>GPMTDWPVYHRIDGPIVMIGFGSIGRGTLPLIERHFAFDRSKLVVIDPSDEARKLAEARGVRFIQQAVTRDNYRELLVPLLTAGPGQGFCVNLSVDTSSLDIMELARENGALYIDTVVEPWLGFYFDPDLKPEARSNYALRETVLAARRNKPGGTTAVSCCGANPGMVSWFVKQALVNLAADLGVTGEEPTTREEWARLAMDLGVKGIHIAERDTQRASFPKPFDVFVNTWSVEGFVSEGLQPAELGWGTFERWMPDNARGHDSGCGAGIYLLQPGANTRVRSWTPTAMAQYGFLVTHNESISIADFLTVRDAAGQAVYRPTCHYAYHPCNDAVLSLHEMFGSGKRQSDW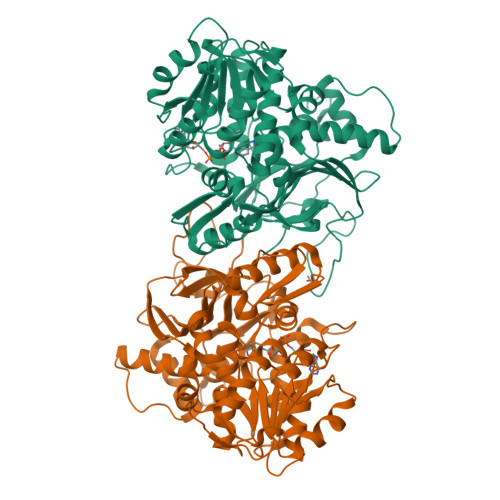RILDETEIVDGIDELGVLLYGHGKNAYWYGSQLSIEETRRIAPDQNATGLQVSSAVLAGMVWALENPNAGIVEADDLDFRRCLEVQTPYLGPVVGVYTDWTPLAGRPGLFPEDIDTSDPWQFRNVLVRD[2x]>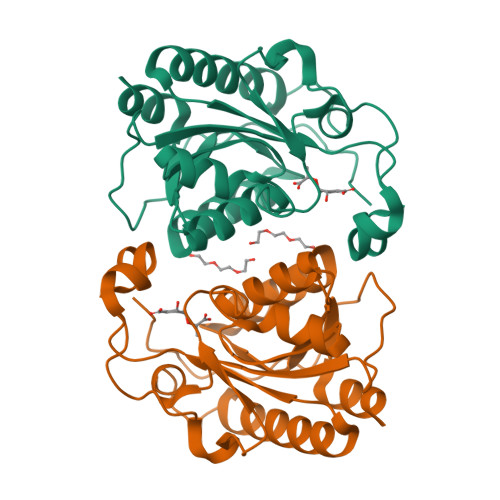 MAIPKIASYPLPVSLPTNKVDWRIDASRAVLLIHNMQEYFVHYFDSQAEPIPSLIKHIQQLKAHAKQAGIPVVYTAQPANQDPAERALLSDFWGPGLSEETAIIAPLAPESGDVQLTKWRYSAFKKSPLLDWLRETGRDQLIITGVYAHIGILSTALDAFMFDIQPFVIGDGVADFSLSDHEFSLRYISGRTGAVKSTQQACLEIAAQHSKLTGLLEHHHHHH>[4x]MASWSHPQFEKGADDDDKVPDPTSAIGVLTSGGDAQGMNAAVRAVVRMGIYVGAKVYFIYEGYQGMVDGGSNIAEADWESVSSILQVGGTIIGSARCQAFRTREGRLKAACNLLQRGITNLCVIGGDGSLTGANLFRKEWSGLLEELARNGQIDKEAVQKYAYLNVVGMVGSIDNDFCGTDMTIGTDSALHRIIEVVDAIMTTAQSHQRTFVLEVMGRHCGYLALVSALACGADWVFLPESPPEEGWEEQMCVKLSENRARKKRLNIIIVAEGAIDTQNKPITSEKIKELVVT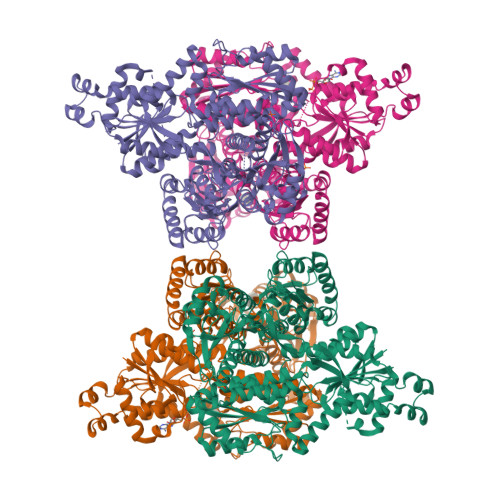QLGYDTRVTILGHVQRGGTPSAFDRILASRMGVEAVIALLEATPDTPACVVSLNGNHAVRLPLMECVQMTQDVQKAMDERRFQDAVRLRGRSFAGNLNTYKRLAIKLPDDQIPKTNCNVAVINVGAPAAGMNAAVRSAVRVGIADGHRMLAIYDGFDGFAKGQIKEIGWTDVGGWTGQGGSILGTKRVLPGKYLEEIATQMRTHSINALLIIGGFEAYLGLLELSAAREKHEEFCVPMVMVPATVSNNVPGSDFSIGADTALNTITDTCDRIKQSASGTKRRVFIIETMGGYCGYLANMGGLAAGADAAYIFEEPFDIRDLQSNVEHLTEKMKTTIQRGLVLRNESCSENYTTDFIYQLYSEEGKGVFDCRKNVLGHMQQGGAPSPFDRNFGTKISARAMEWITAKLKEARGRGKKFTTDDSICVLGISKRNVIFQPVAELKKQTDFEHRIPKEQWWLKLRPLMKILA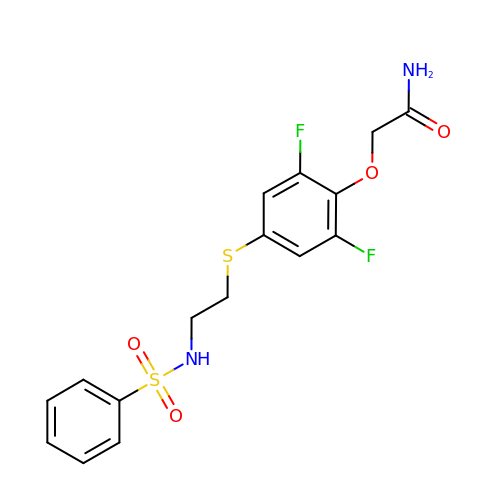2-[2,6-difluoro-4-({2-[(phenylsulfonyl)amino]ethyl}sulfanyl)phenoxy]acetamide | C16 H16 F2 N2 O4 S2 | GTACSIONMHMRPD-UHFFFAOYSA-N>[3x]SGLVESGTLWDHYTLNILEANETQRGTLRVATQVEAAAGTLDNVLITPKKLLGTKSTEAQEGVIKVATQSETVTGTSANTAVSPKNLKWIAQSEPTWAATTAIRGFVKTSSGSITFVGNDTVGSTQDLELYEKNSY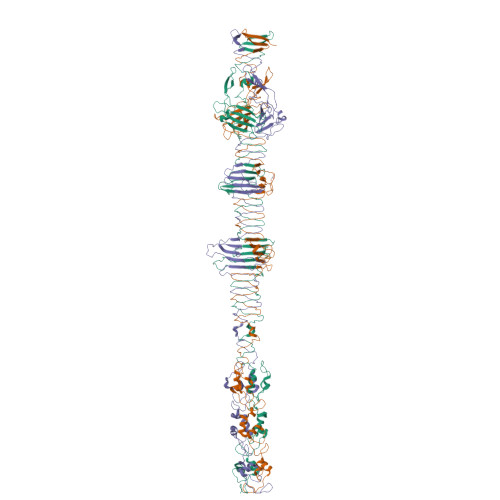AVSPYELNRVLANYLPLKAKAADTNLLDGLDSSQFIRRDIAQTVNGSLTLTQQTNLSAPLVSSSTGEFGGSLAANRTFTIRNTGAPTSIVFEKGPASGANPAQSMSIRVWGNQFGGGSDTTRSTVFEVGDDTSHHFYSQRNKDGNIAFNINGTVMPININASGLMNVNGTATFGRSVTANGEFISKSANAFRAINGDYGFFIRNDASNTYFLLTAAGDQTGGFNGLRPLLINNQSGQITIGEGLIIAKGVTINSGGLTVNSRIRSQGTKTSDLYTRAPTSDTVGFWSIDINDSATYNQFPGYFKMVEKTNEVTGLPYLERGEEVKSPGTLTQFGNTLDSLYQDWITYPTTPEARTTRWTRTWQKTKNSWSSFVQVFDGGNPPQPSDIGALPSDNATMGNLTIRDFLRIGNVRIVPDPVNKTVKFEWVE>[2x]MNIEQLEKENKLLTLGRN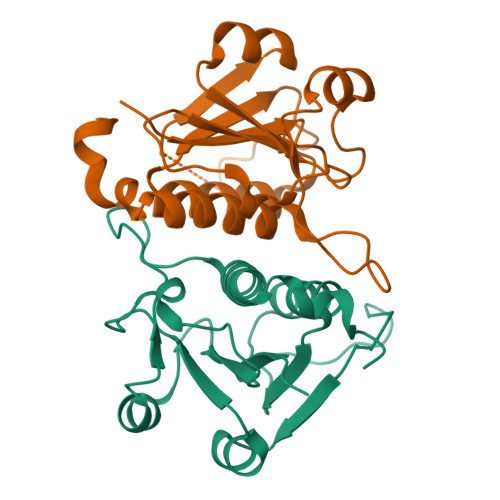HVVLFQPQIPANTGNIARTCAATNTSLHIIRPMGFPIDDKKMKRAGLDYWDKLDVHFYDSLNDFMNICSGKLHLITKFANKTYSDENYDDSEHHYFLFGREDKGLPEEFMRQHSEKALRIPVNDQHVRSLNLSNTVCMIVYEALRQQDFIGLELSHTYAVDKLK> GPLSVAPEMDIMDYCKKEWRGNTQKATCMKMGYEEVSQKFTSIRRVRGDNYCALRATLFQAMSQAVGLPPWLQDPELMLLPEKLISKYNWIKQWKLGLKFDGKNEDLVDKIKESLTLLRKKW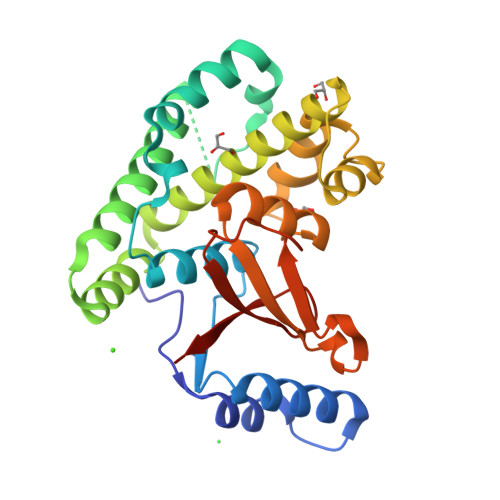AGLAEMRTAEARQIACDELFTNEAEEYSLYEAVKFLMLNRAIELYNDKEKGKEVPFFSVLLFARDTSNDPGQLLRNHLNQVGHTGGLEQVEMFLLAYAVRHTIQVYRLSKYNTEEFITVYPTDPPKDWPVVTLIAEADRHYNIPVRVCEETSL Small Heat Shock Proteins (sHSPs) are ATP-independent chaperones which prevent irreversible protein aggregation by binding to misfolded substrate proteins. Most sHSPs exist as large oligomers which undergo drastic rearrangement or dissociation into dimers upon activation during stress, in order to execute their chaperone function. Aggregation Suppressing Protein A (AgsA), an sHSP from the pathogenic bacterium Salmonella enterica has been reported to form dynamic oligomers. In line with the current understanding of sHSP structure and function, our results show that in vivo, the wild type protein exists in an equilibrium between two oligomeric states: 18-mer and 24-mer.

The construct AgsA:DelC formed only 24-mers in solution. AgsA:DelC, differing from AgsA:DD only in the N-terminus, formed 24-mers similar to those formed by M. jannaschii Hsp16.5 (MjHsp16.5). Cubic crystals of AgsA:DelC in the I23 space group diffracted to 4.1 Å resolution. The application of crystal symmetry on the MR solution of a dimer in the ASU yielded an octahedral 24-mer, similar to the assembly of MjHsp16.5 and S. tokodaii Hsp14. Though the search model lacked both termini for both protomers, successive rounds of refinement yielded clear density into which we could build the C-terminal extensions of both subunits. These termini containing the IXI motifs (residues 143–145: Ile-Ala-Ile), bind in the hydrophobic groove present between strands β4 and β8 of a neighbouring dimer related by a crystallographic 2-fold axis. As observed for MjHsp16.5 wild type and its N-terminal variant, this AgsA oligomer is also charged on the outside and hydrophobic inside. The C-terminal extension in the AgsA:DelC construct forms crucial interactions to enable its assembly into a 24-mer. Constructs possessing an intact N-terminal domain (AgsA wild type and AgsA:DelC) were better at preventing the aggregation of chemically denatured lysozyme.

>[2x]MMALRTLSALPVFADSLFSDRFNRIDRLFSQLTGDTPVAATPAYDLQKRDANNYLLTVSVPGWKEEELEIETVGGNLNITGKHTEETVEDQTHWIYRGIRKADFQLSFSLPEHAKVNNAKLEQGLLLVEIYQEIPESEKPKKIAIES>[2x]MGHHHHHHMIEENLKQKIHDKFVAAKKN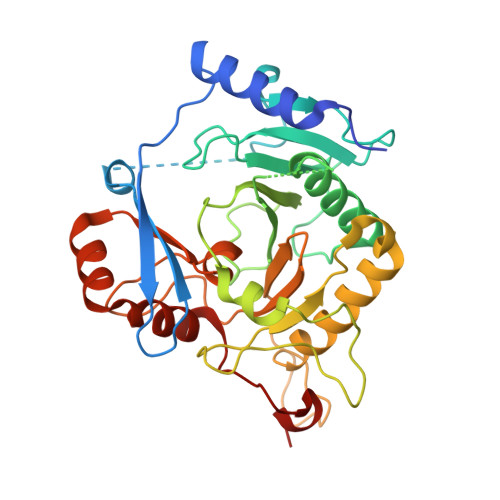GHLKVTHAESKKLKDPQTTTQYWVTFAPSLALKPDANKNSDSKAEDPFANPDEELVVTEDLNGDGEYKLLLNKFPVVPEHSLLVTSEFKDQRSALTPSDLMTAYNVLCSLQGDKDDDVTCERYLVFYNCGPHSGSSQDHKHLQIMQMPEKFIPFQDVLCNGKDHFLPTFNAEPLQDDKVSFAHFVLPLPESSDQVDEDLLAMCYVSLMQRALTFFQDWTNESPELTKSYNVLLTKKWICVVPRSHAKSGPPLMLNINSTGYCGMILVKDREKLENLTEDPHLVDKSLLQCGFPNTAGQKPTEYHY>[2x]MSTRKAVIGYYFIPTNQINNYTETDTSVVPFPVSNITPAKAKQLTHINFSFLDINSNLECAWDPATNDAKARDVV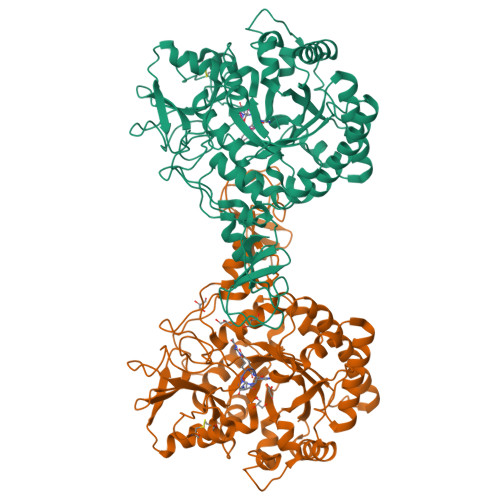NRLTALKAHNPSLRIMFSIGGWYYSNDLGVSHANYVNAVKTPASRTKFAQSCVRIMKDYGFDGVDIDWEYPQAAEVDGFIAALQEIRTLLNQQTITDGRQALPYQLTIAGAGGAFFLSRYYSKLAQIVAPLDYINLMTYDLAGPWEKVTNHQAALFGDAAGPTFYNALREANLGWSWEELTRAFPSPFSLTVDAAVQQHLMMEGVPSAKIVMGVPFYGRAFKGVSGGNGGQYSSHSTPGEDPYPSTDYWLVGCEECVRDKDPRIASYRQLEQMLQGNYGYQRLWNDKTKTPYLYHAQNGLFVTYDDAESFKYKAKYIKQQQLGGVMFWHLGQDNRNGDLLAALDRYFNAADYDDSQLDMGTGLRYTGVGPGNLPIMTAPAYVPGTTYAQGALVSYQGYVWQTKWGYITSAPGSDSAWLKVGRVA;>RPSHX[2x]>RPWQ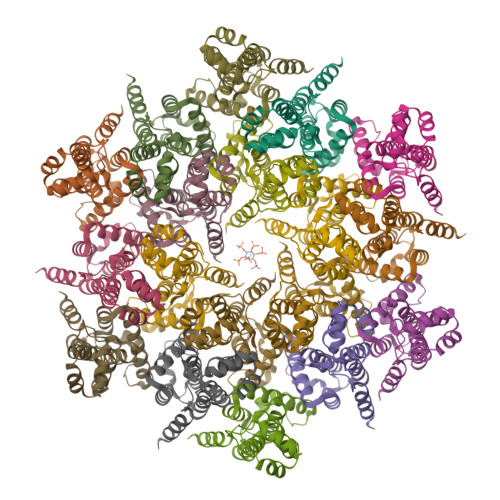MKDLQAIKQEVSQAAPGSPQFMQTIRLAVQQFDPTAKDLQDLLQYLCSSLVASLHHQQLDSLISEAETRGITGYNPLAGPLRVQANNPQQQGLRREYQQLWLAAFAALPGSAKDPSWASILQGLEEPYHAFVERLNIALDNGLPEGTPKDPILRSLAYSNANKECQKLLQARGHTNSPLGDMLRACQTWTP[18x]> MSAMNARQGILSLALKDKPALYSAYMPFVKGGGIFVPTPKRYMLGDEVFLLLTLPDSSERLPVAGKVIWTTPAGAQGNRAA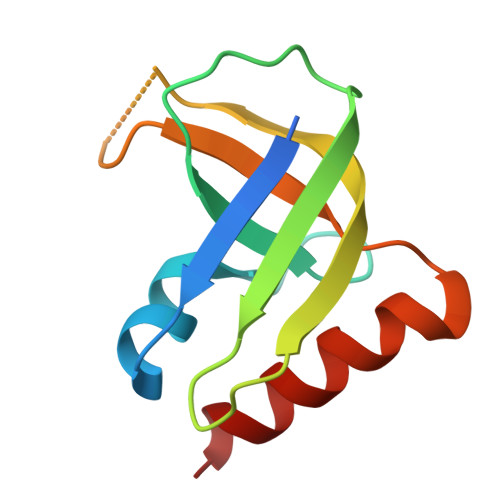GIGVQFPDGPEGEAVRNKIETLLAG> MAFEDRDPTQFEERHLKFLQQLGKGNFGSVEMCRYDPLQDNTGEVVAVKKLQHSTEEHLRDFEREIEILKSLQHDNIVKYKGVCYSAGRRNLKLIMEYLPYGSLRDYLQKHKERIDHIKLLQYTSQICKGMEYLGTKRYIHRDLATRNILVENENRVKIGDFGLTKVLPQDKEYYKVKEPGESPIFWYAPESLTESKFSVASDVWSFGVVLYELFTYIEKSKSPP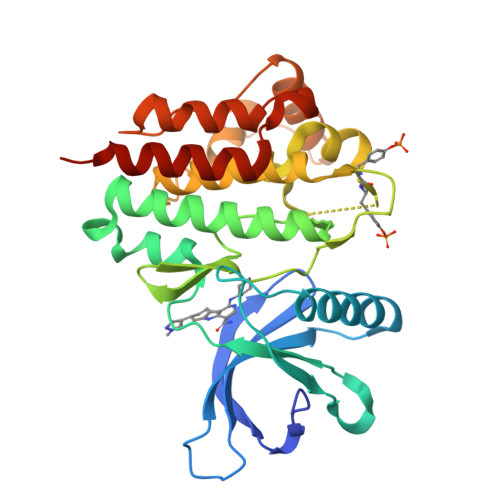AEFMRMIGNDKQGQMIVFHLIELLKNNGRLPRPDGCPDEIYMIMTECWNNNVNQRPSFRDLALRVDQIRDNMAGLVPR>APITAYSQQTRGLLGCIITSLTGRDKNQVDGEVQVLSTATQSFLATCVNGVCWTVYHGAGSKTLAGPKGPITQMYTNVDQDLVGWPAPPGARSMTPCTCGSSDLYLVTRHADVIPVRRRGDSRGSLLSPRPVSYLKGSSGGPLLCPSGHVVGIFRAAVCTRGVAKAVDFIPVESMETTMRSPVFTDN[2x];>[2x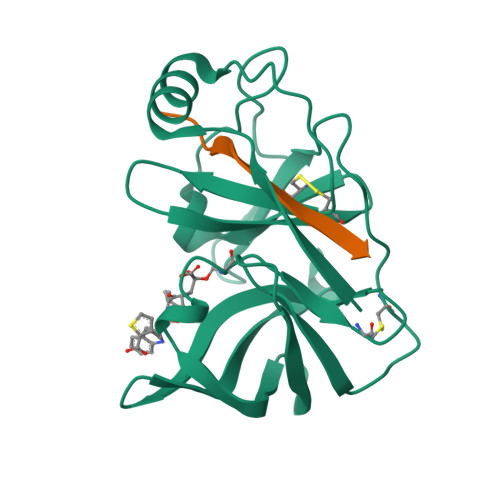]KGSVVIVGRIILSGRK> MGPCDIYEAGDTPCVAAHSTTRALYS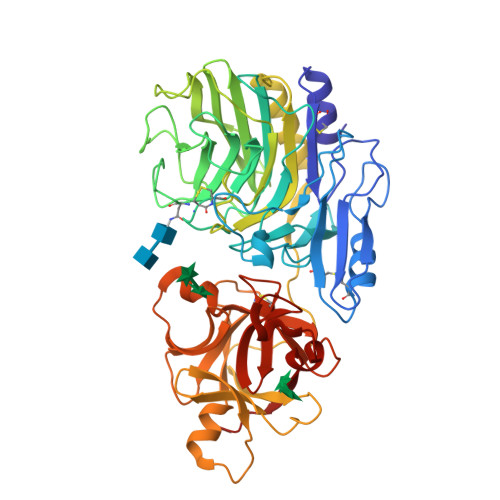SFSGALYQLQRGSDDTTTTISPLTAGGIADASAQDTFCANTTCLITIIYDQSGNGNHLTQAPPGGFDGPDTDGYDNLASAIGAPVTLNGQKAYGVFMSPGTGYRNNEATGTATGDEAEGMYAVLDGTHYNDACCFDYGNAETSSTDTGAGHMEAIYLGNSTTWGYGAGDGPWIMVDMANNLFSGADEGYNSGDPSISYRFVTAAVKGGADKWAIRGANAASGSLSTYYSGARPDYSGYNPMSKEGAIILGIGGDNSNGAQGTFYEGVMTSGYPSDDTENSVQENIVAAKYVVGSLVSGPSFTSGEVVSLRVTTPGYTTRYIAHTDTTVNTQVVDDDSSTTLKEEASWTVVTGLANSQCFSFESVDTPGSYIRHYNFELLLNANDGTKQFHEDATFCPQAALNGEGTSLRSWSYPTRYFRHYENVLYAASNGGVQTFDSKTSFNNDVSFEIETAFAS>[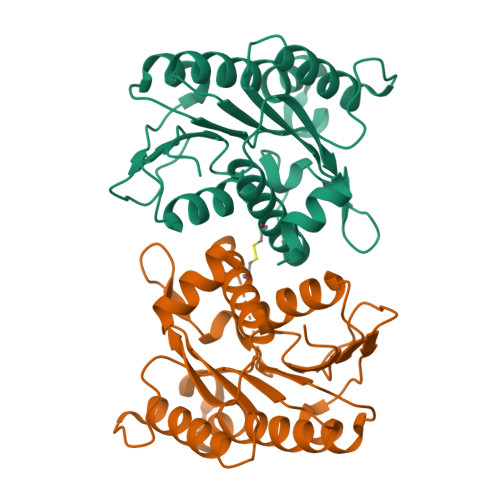2x]MHSTPKRVLLAGATGLTGEHLLDRILSEPTLAKVIAPARKALAEHPRLDNPVGPLAELLPQLDGSIDTAFCCLGTTIKEAGSEEAFRAVDFDLPLAVGKRALEMGARHYLVVSALGADAKSSIFYNRVKGELEQALQEQGWPQLTIARPSLLFGPREEFRLAEILAAPIARILPGKYHGIEACDLARALWRLALEEGKGVRFVESDELRKLGKGS Saccharomyces cerevisiae prevents uncontrolled retrotransposition of Ty1 subfamilies using distinct mechanisms: canonical Ty1 is inhibited by a self-encoded restriction factor, p22/p18, whereas Ty1’ is inhibited by an endogenized restriction factor, Drt2. The minimal inhibitory fragment of both restriction factors (p18m and Drt2m) is a conserved C-terminal capsid domain. Although the crystal structures of p18m and Drt2m are similar, three divergent residues found in a conserved hydrophobic interface direct restriction specificity. Structural and genetic analyses of p18m reveal that p18m and Ty1 Gag interact through a hydrophobic region that is shared between both proteins, termed the Dimer-1 interface. These observations suggest a lattice-poisoning model of restriction by p18m in which the CTD binds full-length Gag and forms dead-end intermediates in VLP assembly.

Given that Ty1’ CA and Drt2 also encode p18-like domains and to understand if they had the same Dimer-1 properties as p18m, we expressed Drt2m and the equivalent residues in Ty1’ CA-CTD (Gag coordinates M259-Q351) and determined their crystal structures. We observed p18m higher order aggregation through a weaker Dimer-2 interface that was ameliorated by introduction of a Dimer-2 suppressing mutant (F323S). Therefore, we included F323S in Ty1’ CA-CTD constructs and in Drt2m F323S/Y329S (SS) for crystallographic analyses and F323S/Y326S/Y329S (SSS) for biophysical analyses. Inclusion of serine substitutions reduced the aggregation tendency and improved solubility necessary for structural studies. The asymmetric unit of wildtype and Ty1’ CA-CTD (F323S) crystals both contain two monomers arranged through a single Dimer-1 interface and the Drt2m(SS) crystals contain four Drt2m(SS) monomers arranged as two dimer-pairs through Dimer-1 interfaces. Inspection of the structures reveals all helical domains with arrangements and packing resembling that of Dimer-1 observed in p18m and confirm that the F323S mutation does not alter interactions at the Dimer-1 interface. 3D comparison of the Ty1’ CA-CTD (F323S) and Drt2m(SS) dimers also reveals the strong similarity with RMSD of 0.5 Å over 160 Cα backbone atoms. By contrast, in Drt2m and Ty1’ CA-CTD, it is the V266 sidechain on helix α1 that closely packs against F312 on helix α3 and because of the greater steric bulk of the V and F residues the distance between the V266 and F312 Cα atoms is increased to 6.8 Å. Concurrent with the increased spacing in the VTF interface of Drt2m and Ty1’ CA-CTD, the side chain of the conserved residue R315 can adopt a rotamer that allows it to swing in and hydrogen bond with T270 which is not possible with V270 in p18m. Thus, this “arginine-flip” mechanism provides a further level of discrimination and specificity between AVL and VTF Dimer-1 interfaces.

>[2x]MQSDTQEVNDITTLATLHYNGSTPADAFEAEVTNILDRLNNNGIPINNKVACQFIMRGLSGEYKSLRYARHRCIHMTVADLFSDIHSMYEEQQPLEH>[2x]GSHMTAVPNPPLPAQDPIVQHLKLTNDQITRIKKLHQQLETD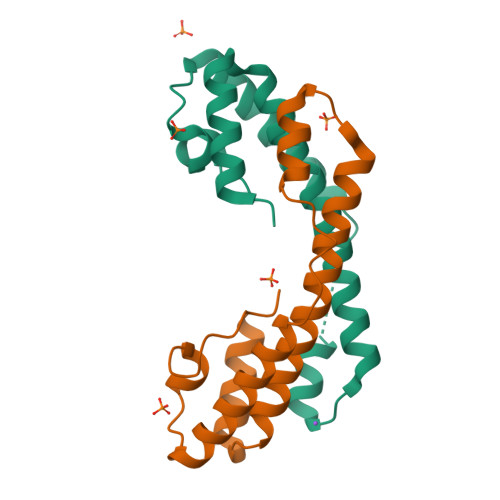VSQISMKGIKDGALIEVIKSGKWDDAAVKQQLAAFSNIEQQARYYRVKYYFDLSKVLTPEQRQQVQQDLAQALE>[2x]MVRRTKEEAQETRAQIIEAAERAFYKRGVARTTLADIAELAGVTRGAIYWHFNNKAELVQALLDSLHETHDHLARASESEDEVDPLGCMRKLLLQVFNELVLDARTRRINEILHHKCEFTDDMCEIRQQRQSAVLDCHKGITLALANAVRRGQLPGELDAERAAVAMFAYVDGLIRRWLLLPDSVDLLGDVEKWVDTGLDMLRLSPALRK

We chose TtgR, a ligand-inducible aTF belonging to the diverse TetR-like protein family, as a target for computational engineering of ligand specificity. TtgR is a 1-component transcriptional system and represents the simplest molecular mechanism for converting biophysical interaction between inducer and protein into a complex biological response like transcription. When induced, ligand-binding allosterically lowers affinity for DNA, thereby allowing transcription. TtgR is a compact, dimeric, all-helical transcription factor with a large cavity between five angled helices forming the ligand-binding pocket.

To understand the structural basis of TtgR-ligand interactions, we solved high-resolution crystal structures of quadruple mutant (resveratrol-bound and apo) and wild-type TtgR (resveratrol-bound) at a resolution of 1.9 Å or better. In wild-type TtgR, the four mutated positions (C137, I141, M167, and F168) are located approximately in the center of the binding pocket and make nonspecific van der Waals interactions with resveratrol. Other neighboring residues N110, D172 and H114 make specific hydrogen bonds that stabilize resveratrol in the vertical orientation. Although both naringenin and resveratrol bind in the vertical orientation, only N110 is able to make a hydrogen bond with both naringenin and resveratrol. The ability of wild-type TtgR to bind multiple ligands likely arises from the nonspecific interactions made by the nonpolar amino acids in the binding pocket. The DNA-binding domains of the resveratrol-bound quadruple mutant and the resveratrol-bound wild type are extremely similar with an all-atom RMSD of 1.0 Å. The four mutations do not substantially change the volume of the pocket (215Å3 in wild type compared to 234 Å3 in the quadruple mutant) or the surface area of the pocket (184 Å in wild type compared to 186 Å in the quadruple mutant). The structural basis of ligand specificity relies on the I141W substitution to create a steric barrier to prevent binding in the vertical orientation, which is observed in wild-type TtgR for multiple ligands.> NEGCAPLTGKESGMDIGRSSTERCLPGANPLQDQQWYLLNSGQDGFSARGGIAGNDLNLWWAHRTGVLGQGVNVAVVDDGLAIAHPDLADNVRPGSKNVVTGSDDPTPTDPDTAHGTSVSGIIAAVDNAIGTKGIAPRAQLQGFNLLDDNSQQLQKDWLYALGDSNASRDNRVFNQSYGMSVVDPRSANSLDQSQLDRLFEQQTLKAQGAAYIKAAGNGFNKIAAGGYVLNRTGNGPKLPFENSNLDPSNSNFWNLVVSALNADGVRSSYSSVGSNIFLSATGGEYGTDTPAMVTTDLPGCDMGYNRTDDPSTNRLHGNSQLDASCDYNGVMNGTSSATPSTSGAMALLMSAYPDLSVRDLRDLLARSATRVDAKHQPVMVSYTSSTGKVRDVKGLEGWERNAAGM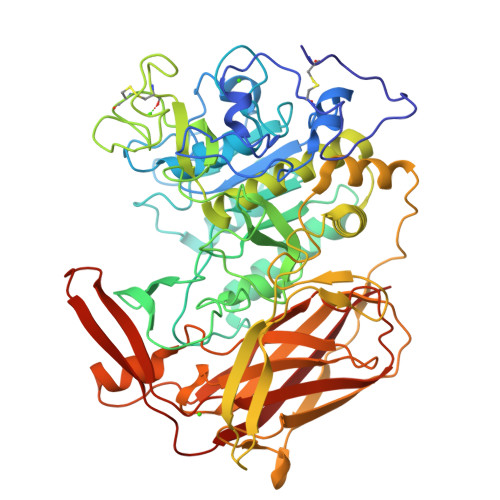WFSPTYGFGLIDVNKALELAANHQPLPPLVQLPWQKINVTGSAAAIADVGNSPTSSTTRIATPLTVEAVQVMVSLDHQRLPDLLIELVSPAGTRSILLSPFNSLVGQSLDQQQLGFVRTKGLRDMRMLSNKFYGESAQGTWRLEVTDVANGTRQVSLLNRETRERTTLTERNNRQPGKLISWSLRVLGHDANRS Phosphoramidothioic O,O-acid | H4 N O2 P S | 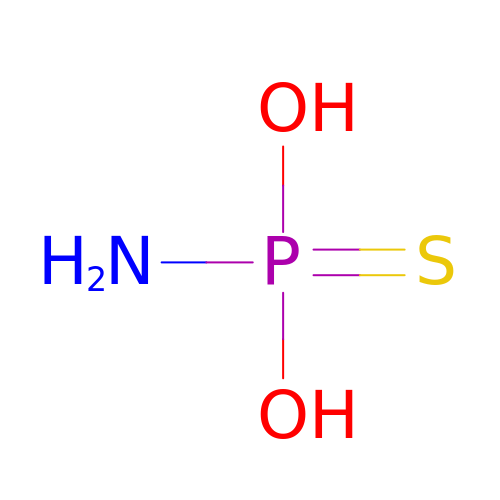RJBIAAZJODIFHR-UHFFFAOYSA-N> MSSKPTDRGQQYKDGKFTQPFSLVNQPDAVGAPINAGDFAEQINHIRNSSPRLYGNQSNVYNAVQEWLRAGGDTRNMRQFG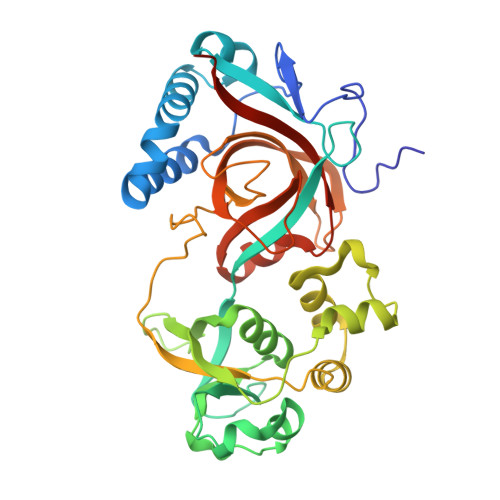IDAWQMEGADNYGNVQFTGYYTPVIQARHTRQGEFQYPIYRMPPKRGRLSSRAEIYAGALSDKYILAYSNSLMDNFIMDVQGSGYIDFGDGSPLNFFSYAGKNGHAYRSIGKVLIDRGEVKKEDMSMQAIRHWGETHSEAEVRELLEQNPSFVFFKPQSFAPVKGASAVPLVGRASVASDRSIIPPGTTLLAEVPLLDNNGKFNGQYELRLMVALDVGGAIKGQHFAIYQGIGPEAGHRAGWYNHYGRVWVLKTAPGAGNVFSG>[2x]CLAEGTRIFDPVTGTTHRIEDVVDGRKPIHVVAAAKDGTLHARPVVSWFDQGTRDVIGLRIAGGAIVWATPDHKVLT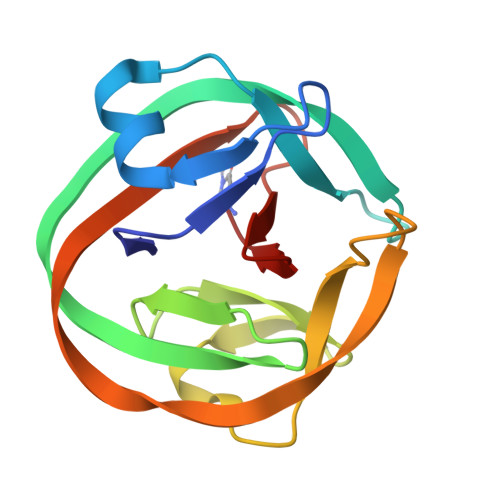EYGWRAAGELRKGDRVAVRDVETGELRYSVIREVLPTRRARTYDLEVEELHTLVAEGVVVHN> KYSKRIAWMKTTICDSLQLKDMIVEESFQYEKNKNLLEQFLSGEGLNKIFAYYQVQEQAQNDDIKDTGAQDPVLFFTTGDLEKIQDKAVWFLRITNPADDKKKASQQDGNDNDIIFGEITPNTVPMLNALMESVYSRQIDHIITEKIQFWGVAEEEQVLEFQQHSNKFSSEVREAINLMSPGTEHFKLDYEAISGLSESEKMQHYEMKFNEWINLISSQLNDDSEVRKDEKDAGPATELIYWRSRMQKITNWSEQLKSKDFQIVKASLQRHKNHDNQRPRGDESLSKLMMEYNRLDLLLTDKLNEAKDNVKYLTTLEKFIEPLYNGTPQQIIDTLPALMNAIKMIHTIARFYNTTDKMTGLFIKITNQMIKNCKDRILNKKDNGDNPSLYKMIWEQDPAELIEVLGSCIKLYCEYKKCYNDTKEKVADMPKGKTFDFSDAQIFGKFDTFVRRLQKLIEIFSNIQQFNALAKHNLEGMDVLTNKFKKIIDDFKKKGHNLLDTANNKFDRDWVEFNVEISHLDGELQNFIDNNFNRFRNIEYSLKLLHKFQSTIKRDSLKHNLTSRYNAILHNYATELDTIQRVFQDQKSNPPLVRNMPPEAGKIIWARHLFQKITGPINIFPENVINSTEIRRYYGSYNTLGKQLTIYEMWFYQDWVNKIEQSKAALQATLIVRHDENKKLYVNFDLEIMQLIREAKCLDRQGIEIPESARIILLQEDKFKTYYNELLYALKEYERINSKIKPICKNLLLPHIEDLDLKLRPGMVTLTWTSMNIESYLYYVHQGLKKLEQLIINVNDIIENRIENNLKTVSKVVLVHLPQDTKPLSLDSFVQLQEEYINSKTDFLTSKNVEVERAVDDLLQTIMLYPLDPHVDPVLPEETKRIKRYYFWYFYQALLNSTQNSLNAMKYRVCGKKIPGANTLQNLKPFFQVEVQLNGDKVTLNPSLQEIQKSINRAATAVLRCSKHLYNWDQQNKDSTDKATFYDMIACDKEIVKVILLLTGSIQGTKNKVNEFLSGFTKFEWLCKESIQESIKKFSKNGPTLQNYEDQLKKFSQIEEEIEKIVPTYKIGAMELMTHNICTSLSTWAKEWKLQYSQDLHKRARQLLDSLTEQTKMLSTKLSKPVKDIDSLGYVMETLEQIRKEQAEIDMKFNPVQEMYSLLDNYLPGGITDKDEMDARSLLRRNWDILIQQAEIKGKEYQHKQAIYLKELKQSIKDFTNQVSIFRRDYEKNGPMVEGISPAEAMERLRRFEDEYDVKYQMYKINARGENLFGLQNQKYPELEKTDAEIKNLNKLYNLYDSVIKNIQQFKEKSWQDVSKDDLAKMEEDAGKYGEQCSRLPKDLKEWQAYRDLKNYIDSLREQLPLIISLKKPSIMPRHWEKIKEITNTKLNYENPDQFYIEEIMGAKLLDFREDIEDITESADKQLKIRTGLDEINLYWNDMQFQFGIWGKRDVPCMLNGLIVGTILERLEEDQLQLSTFNSQRHVTPFKAEVENLIRTFSDVNDTLDMWVKVQKLWTSLEPVFTGGDIARQMPLQAKQFQGIDKNWMKIMEKAVETKKVIPCCQNDMLKDFLPDLNRKLEDCQKMLEAYLEGKRKKFPRFYFVSNPTLLKILSQGSEPTSIQEDFEKLFDAITKVTFESAKDKKNPALKQITQIQQVIGRNEENISLTGYYVKCEGNIEDWLKKLEQNMQQTLKDIASAAAQQVFQVGLKEFVSSQASQIALLGLQILWTSKVNEGLERLSRNERNAMDIKRNEIKEHMNILSSMCLEDLNGAVERTKVETLVTIQVHQKDISMDLKCKDVNDFEWQKQTRIAWKTDIDECIISITDWDSPYSYEFLGAKERLCITPLTDRCYITLAQAMSMYYGGAPAGPAGTGKTETVKDLGRTLGVFVVVTNCSDQHRYRDMAKIFKGLVQSGLWGCFDEFNRIDLEVLSVVAMQVESITTARKQHMKKFMFPEEEIEIELIPTVSYFITMNPGYAGRQELPENLKVLFRGVSMMVPDREIIIKVKLASVGYLQIDLLAKKFNVLYRLCEEQLSKQRHYDFGLRNILSVLRTAGNTKRQEIKSDEEMLLMRSLRDMNLSKLVADDIPLFNGLLADIFPKLKEVPKKLYPDVEKKIPEEINAESYLINTPSFQLKIIQLYETCLVRHGFMLVGPTGSGKSTIMKILTEVLTKLGSPHKIVIMNPKAITAEQMYGVKSEISDDWIPGVFSTIWAKSNNRALKHTTWITCDGPVDAIWIENLNTVLDDNKILTLANGERIAMTENCKVVFEVENLNNASPATVSRCGQVYVSPTDLGYEAVIEGWIRNRKASGRAEESDKLGNILRKYLINMRFIELQSKECKEPMMDTSPVISVINILNLLTGCLQYFVQTQRTLSEQEYEKFIVYSMAWAIGGIYEAQDRVRFHELLLAKNAPIPQKGKENETVFDYYVSQDYLDWKICSPEEWVPPQSLQFSQLLLPTLDSFRAEMLLNFILTQPKSHTCSNSALLIGGSGTAKTSSVLLYCNKFDPQKMLFKRTNFSSATSPFMFQSTIEAECDFKVGKEFAPPGNKMMTIFIDDMSMPFVNKWGDQITLELVRQLIETGGFYMLDKTQRGNQRKMKNLQYIGAMNHPGGGRNDIPNRLKRQFFIFNMILPLSIEGIYGPIIKHMFKQKYFSDSTYKVIESLTSATIALWNKVKSTMLPTPAKFHYVFNMRELSRIFKGILTCKKDTINDAPKSMKIKPELFLVGLWRHEAERVLADKLVNNKDKDTVMGYIQEVSLESFSQIENEILEKYSSEKTFLFCDFLRPDVINEDGIIEEEAPKIYEAIDSLTELRKRCNFLLSFYNDRNPSKKMPLVLFDDALKHLLRISRIIRQPRSSGLLVGVGGSGKQSLTRLAGFIGKNLIQQIIVTKTYSDKDLKEDIKKGFDDAGHLGKQVTFLMTDSEVKKEEFLEYINMVLSTGEIPNLLAKDEREVWLGDISQAYCKEKNLGNIDPPQSELWTYFVDRVRDNFHIMLCFSPVGQKFRERARKFPALFNECTIDWFLPWPEEALVSVAETFIKNFDKLDTKEETKQELMKHMGNVHLMVNEICDEYYQKMRRQVYVTPKSFLSYLNSYKTLYIEKYDELDQQEESFKIGLNKIQEATITINQMEISLKEEEIQLNEATEKTNQLLANLDKESKKANQKGEEVAATNKQCEIQAEQISKEKEEAERELEAALPALRRAQEAVDSIESKDIVELKANKKPLDIIKYIMNAVLVFFKARLIPIQIEERVFNKKEGKAVLFLKESYDESGIQTLGDMNFMKKLKEFEKDSINEETIELLEPYLNQSEDWFNDTFATKASKAAAGILKWAFAIYEYHQKSKIVKPKRIQVAIAEGRQAIALKELEKAREDLAQIQAYIKNLKDVYTKQMEEKNELEMKAAKTKKKINTARTLITSLSGEKDRWGKGAQDISDQKRKLVGNVSLSTAFISYCGPFNAEYRNKLAQQRFVVDMKKRGVPVTPGLELTSFLIDDATIGEWNLQGLPKDDLSIQNGIMVTNSARYPLFIDPQGQGQNWIRNKLSASIIPERCITTLSHPKFKDMFLKYCMESGLTLIVENIENEVDPMMDPVLERQIIVKGKTQFVNVAGTEMELSKEFKLFMTCRLANPSFSPELSAKTTIIDFTVTQSGLEQQLLGKVISKEQKALEDSLNQLLADVNQNQKDLQRLDKNLLERLINSQGNLLDDTELMDVLNNTKTQAKEVAAKLIDAEIKTKEINEKREQYRPVAIRGSAIYFTMIEVSLVNWMYNSSLEQFLKLFIESIDLSEKAQLPSNRVKNIISFLTFHVYRYVNRGLFEKDKITFILMMAFKILTTAGTISSGDVSLFLKSGDALDIKSERQKQISYLEDNQWLNILALSKHTFSGQTLPFFKELPDLISRSENQWRNWIDKNDPENFPIPDFAESINQEKEIGSFISLCLVRSLRNDRTLIATQNFISNVLGKEFTDPISYPIEGIWQESSNMDPVLFLLSAGADPTSSIDELAKKKKKFPCEKVSMGEGQERVARQVIMKGFVEGGWVILQNCHLGLKFMEEIETLVSPINQIHEDFRLWITCEQHPKFPLGLLQKTLKVTNEPPKGLKAGLYKTFTTIITQEFIDKVDHSNWRSLIFTICFLHSIVIERKKFGPLGWCVPYEYNYSDLEASLLYIEKYLTNLMSTPQPNSHNLPISMNVVRYMICEVQYGGRITDDLDRELFITYGETYLKDGIFGNDYFFYDIMVDGSGQKFKYRIPQNPSAELIKYQEYIAKVPTVDNPEVFGLHSNADLTFRLKESKEMINTVMETRPKDSSVGGGKTREEIVQDKAKDMLKNLPPDYNDVEVRELVSKLGGPNPKTSTERGMTVPLNIFLYQEVTRMQRVIGLVRKTLQDTILAIDGQIIMTPEILEAINAIYDAKVPNSWLYDPSGAEISWLLPNLGSWSTSLSDRNKQLNDWLRSGQRPILFWLTGFFNPQGFLTGMKQEVTRNHKKGDGKGGEAWSLDDVVYSTTVKEREKEKDIEQPPAEGVYIKGLYLEGCKWSKNGLDDSDPKKIFADLPILHVSAINKKKTNEQDRMSNTYLCPVYKYPKRTDKYLIFRVGLPCEGSNNPSHWKLRGVALLCST;> MGDHSQKDSPEDFIINRLSQALGIQKEKIKKSLETAQDDKGEVTNKDEFQGFIQQDNSTNILWVSGQSEKCTFYYGQLPPIDKFKKKGIAVIKLGLHKLTNENVAKDVVVVEITNNLLEHLNSVFNEIMSPVMQNPLNQQGWTDLVAKDLMEKFNNYVAQVYVLLGQIKGKTMLPLPSHKLTSSDTTPDKDKAHVFEGSIITWTKQIKNVLKLEPEQLLKYGNDPGPLAEIEFWQNKRDNLNLIDSQLKSVEVQNILHFLDNNKSTYTTPFTKLQAEVKKARLEANENYRYLFTLKDLFSKLQESQPSDFPTLYELFIPIMHTILLIYNKSKTYNQPPRLVVLIREICNAIISNAQAFVDKDTIFSLIDSKETTEACDKLQVTLDVCSKFKDAYFEYKAKAGGNWKLTSNALFVRLDSFLERCQDILHLTNTIVQFNKLEKIELGGTKGKTLTESIAQIFKEFEEAVQAFTSVSYDIMNIAEKKFDDDFYEFRSKIKELERRLASVITQGFDDYDTIYGRFKLLDNFEGLLTRPIIADELEKKHIVLLEMYKQDLKQVQSIFLEGKQFVDSMHENAPLFLNMPPIAGALTWCKSLRDRIQEPIEKLAQLGQGITEREEYKDVQKLYTSITKSIKDYEDQKILSWEKEVEDSSQDKLKQTLLCKDENDLIKVNFDPSLVRLLKEVKYFLLLRLEVPTTAKDIYTKAETYRTQIVALDMIVDNYNHIKTCLLPVEEPLVKKKIQDMEEEVKPGIEEIRWKSTNIDQFISKSKSIVDQLFETVNKMKDSLQKIHKSLANFNVKIIERKNRPMSPDDYDQFLKAIFSNKLTIVKDNGNQIQKLVKEVLDAVKADKKQNSWKNYNDYVNVIVIEGISTAIQTALLHLNEQINPVFIKRNDISPLFDIRLELGQSGIQFDPEIGESSNQLTVRNTIRNWINDFFNIAGTIQRLDTTMPGDFLQEIRSFFEIKQCLAMITQNLEWIENECNQFRARFDTYSYLWTEDEQISFNRFLDENEPKDEDGKGGDDDEGENTEKQNPLLKGCRAKIPNLDLFDEKITHLKAIQQEISRIKTPEDISWLRINLQPMKTALDARVTRWIRVYTDFLVNQFRTTQKNLLDFIEKTKDGIKKNPADHENLHDKKLLMSVMKVISDVKDVEPRREGIITRMKEMVTKLKKHNVPITEKGTDDPLQQIDNANSNFIEIYGRVFKVKADIIPLQAEETQNIKRDLDIFMKEVESFRKEFMQKLPFDYTESMGYENINNAYDTIMVYYHKLTAIEGRALEYNNLEKAFELQKSNYKQLKDCMNDLKNLKTMWDAIALIHFQYNDWKTKPWRQIKADILLDTNKTLGTQIKNLPKEIRNFKGYNVIVEKVKNMGTVLPLVSALHSEFMEDRHWSQLKQITGTVFDHNSLSFYFEDILALNLYKYENTVNEIVDVAQKEAKIEKKLKNIEQWWSKQVFEFTEYKETKTFASLDNMMEVLDQHSLDLMGMKSQGKYVEFFYDRVEDWREKLGRVDVVVNEWLKVQKNWKILYNIFLLSEDIRMQLPEDTKVFEGVDKEFKDMMSEVSANPSVVEACTIERRDVLVGWSQAIKKCEKALNDYLEQKKKSFPRFYFLSNQSLLTILSNGQNAPKVCEYLGDCFDGLKTLTFEPPANPAETSKVGIGMISKDDEKVPFSSKFICEGAVEHWLLNLEFRMRETLQEILEGAKNTADLWDSGDKPREEWVEGYNAQIALLTTTIVWTEDVGRAFEDLAGGSETAMKECQKLIEVRLENLIKKVRGDLHILERWKIINIITIDVHSRDVVEKFVIQKVSEAESFAWLSQLKFYWENKPDSDMHLRQTLRFPWEKDKNKNKCIIRIVDWFRFYSYEYIGNAIRLVITPLTDRCYITLTQALNLTMGGAPAGPAGTGKTETTKDLGRAIGIPVMVFNCSDQMNKDSMAQIFMGLSQSGAWGCFDEFNRISIEVLSVVSTQVKCVLDALKEKKTKFSFVEEGEIQLQDTVGFFITMNPGYAGRTELPENLKALFRSCAMVVPDLALICENMLMSEGFTMARVLSRKFVSLYMLSRELLSKQKHYDWGLRAVKSVLRQAGKLKRGDPDMPEDPLLMRALRDFNMPKIVTDDKVIFRRLIGDLFPKLDPPTKQNPELKKIVQDTTKKDMGLVAEELFVTKVVQLAEILEVRHCCFVIGPPGSGKTCVWKTLIKSYINSGEDAEYDTLNPKAVTSDELFGAYTKTKEWKNGVIAVIMKNQVKNEEKYKATHMHKWSVLDGDIDPEWIESLNTVMDDNKVLTLVSNDRIFLTPQMRLIFEISNLRNATPATVSRAGVLFINETDIGWMPYMNSWLERSQINILKQQKEMANMPEYPVIDDVAKSVFYRCFQSYFEQNIDVHDKNRVRHICPMVDIAMIQTICTILDALLIQHLPKLKQMKEEDEKQALEAFFIFAGLWAIGGPVGGGQDDSKDMKEFNTVWKGAAKVKFPEQGLCYDYYYDINENKWNTWKVEDYLPNDQPLFSKIYVATIHTTRLRYMIDIHLQRRKPILFIGSAGTGKTAVVRDYLNSTRPEQVSHKTINFSSFTDSLALQKNIESMVEKKNGRNYGSATNKVLICFIDDFNMPYVDKYGTQSPIQLLRLILDYGSIFNREQLEERKFLQDLLFFGCLNQKSGSFTVDLRLQRNFSVFSMYTPSSDVIKTIFGSILNAHLSTIDDKAQKMAFKLVEATYFTFDKILKNTTAFAPSAKRFHYQFNFRELARVCEGICRTTPGQYSGGDQGKLVRLWAHEMKRTFEDRFIANEHVEFFRRYLTEAISKCIGEFPETENPIAEPLIFTGFVAAHQGLDQQYTQCTIPVLKRVLDDKLEEYNEVKAQMNLVLFQQAMEHVSRICRILDMPGNNALLVGVGGSGKQSLCRLSTFINGFEIDQLVVTASFTINDLRNNLQEIYKKIAKPNSIARVFMITDSQIKEEQFLIPINDMLNSGWIFDLFPKEDMDSLVSGVRNEAKGEGVDVNNLTALTSYFLDKIRKNLKVVLCFSPVGDTMRIRSRKFPGIINNTSIDWFHPWPHEALIDVAFRFLEEIEFPTEEIRQSISLNMAKVHSSIDTANEKFLKLERRYNYTTPKSFLELIDFYKKLLTEKRETIQRQIQRYEMGLNILAETQNKVQGLQEELKVKMVEVNKQREETDILIEKVGKESALAEEEQTIANAEEEKTNVAAAEAEKISKEATEALAEALPALRSAEAAVDCLKKPHVTEMKNLGSPPAGVIVTARVVLILFNQGITLNDPDEKVWKKAVTFMNNPQAFIDKVKSFDGENIEPNIIEQSNKIIQDPSKKFNEKDMAGQSYAASKLCAWAVNIVTFNKIFKQVKPLQDAQKQANEILEEKKKELAIVKQRVAELNARVNSLKRQLEEAEARKMIVEQDAARCQSRLSAAENLVNGLAGENKRWTQNVKFLKENIKSMIGDSLLASAFVSYIGAFSAKLRLELWKNTWLPDIIEKGIPITEGIEPLKILTTEAIKSKWKNEGLPADPMSLENAAIITACARWPLIIDPQLQGSTWIRGKQGENLTTISLSQPKWLGALTSSISSGRAVLIEGIQQEIDATLDPLLQRAVKKNGNQLQLEIGGDPIDYDPNFKLFLMTKLINPHFRPEIAAQCTIINFIVTESGLEEQFIAMVVNIEKNELEMAKQDLVKKQNEYAVTLDKLESDLLQSLSEADPATILDNTELIQNLDKTKKTTIEITEQQQKAKVTEAEINIQREHYRVVAAEGSMLYFLVISLSVMDHMYQYSLESFITFFFKAINRTTVRDENRIPTLILNIRQTIYQWISRGLFEKHKLIFLTLIVFRLMQKKIIDVAYEVAEMDFLIKCPARPGVENTLDWLPNISWDQIQGLINLEEFRNFAHQLEKEAPNRFKDWYNELQPEDQKLPLDWKRLDSMPFKKLLVLRCLRPDRMTISLNNFIRAVLPQGDAFVEMDQKLAFSEILESVINEDAESTIPIFFILSPGSDPVKEVEKIAKKKRIEPGKNFFNIALGQGQDEIARRRIEEGNKEGHWVMLQNIHLMPTWLIELEKILDSYSGEAGGGNSEFRLFLSAEPSTGIPIGILDRSIKLTNEPPAGLKANMKRAWTYFSKEEIEDKDPKIKSILFALCFFHSTLIERRRFGPKGWNMSYPFNMGDLRDSYLVMNRYMEQNQGGKVPFNDLIYIFGEIMYGGHIVDDWDRRLCNSYLFNTMHEQLFDELELFPYIEGKGLSFKVPGQNPYEKYIEHIETSLKQETPLAYGLHPNAEIGFRTDQCKTLFNTLLELMPKEQSRDEKSSDIKSSNEMASDLIKQLLEDSELKNKIFNMEEIKNKIDAENKGPYQNVFLQEIEYMNALLSEIVKDLEEIGQGLSGLLTVSENMEMIIESIALSRVPASWQKLAYPSKRGLQSWLANLFQRIEQLNIFRDDPYSIPRVVMISRFFNPQSFLTAIMQVISRAKAYELNKLYIQTEITKRSIEEIEGAAKEGAYVYGFILEGARWDYQLGQLEESKPKEMFSVLPVTYCKAIPLPPEGKEDKSLYQCPVYKTEDRGNTYVFTAQLKTRFPPRKWILAGVAIIMDVEGVSD;> PLVWTQLKQTGTTQPTARSGHTIITVGKTHIMFGGLDNDKNNYKDGKIAPNNQVFTLKLTQNNCEWRQIACQGDVPLPRCYHASCAISADKMLVFGGSYTSNLRFNDTYILKTTSYQWSKPANQISGGEPKNAESKIGAPQPRYGHSATFFEGKVYIFGGHGGINYQRLAFNDLYVLETENFEWTRLEPKGNPPDPRGGHSAAMMANKPQLMIFGGWSFTSQYSNIMIYDIEKDEWVDPEIAHEIPKWNLSGIMAPSIPSWKYFIFGGSVGSFEEGGNRTNSRFVDDSFVLDIDTLSWSSINLEADETSKAVCKPRPRESASIFYDSGESRAIVFGGWANNWLNDLWALNVSTITGPPIFSIKPALGPLTGKTKVLIEGDGFKDTQNISVKFSGGKLEKEVNGTFVNEKEISCETPTFDYPRSVEVTVCMNKGDYTITKSAFTYNTKADKTIAYGPGLLTENLIGVQTTIVIQARNGSDEFVVTIRNPAKIKKEEEVKEGDKANTKNTIKEDEEEEGEDEEENKKKKEAEKNDLTGSAVMNYISKQLKDIQEFIENTKENIEIRNKNISELINVMINLEKVRVKNDDDVLTLDTVEEMLNFLKKKKDSDIKKCKKLQEEWKNLAKMAQAVKKDIQNPVKTESDKTKENIKKFEEITLKEYANSLKKESFFIYKTGVSESFKRIGEVKQKVDEFEVQLNQYEDFARIGSKKLMEQIRTDVSSVEKLWVRIEISEKTMDEYKKMKWGSINSMDMEDEIKKLRKALTDLRGIDKRSNAFIGITEELKKWATFLPLLGELKDPSMNSEDGRHWKKLKDLVKKEFDVSQELMLEIIWDLKLFDYKDGIEEITDQAKQELKMEKALKKIIDFWRDIEFELVQHKNTDIHTLKMSEENFETLEDHQLQINNMLLSKYVAYFEKEVEKWKYDLGSVYDVVQLLLEVQKTWSFLENLFEVKRELPNESAQFVGIDKDMKEIMQKGCDIKNCLKFCTIEGMLKRLENIQAQLKVCEKALNEFLDSKRRAFPRFYFVSVNDLLDILSNGNSPAKINRHMSKIFQAIDNLQLKEDSSGGRPTLKMISCVGTEEVDFSSPRLLQGKVESYLKDVIDTMIGTLKSVANSSFKNFQSMTRKEWLKSDPSQITLLVNNIIWSKAVEDCFLKLQSGDINAMKLFLDESIKQLTELIGMVQGDLSKPLRQKIMCLITIDTHSRDVVHRLINEHVRKAEEFQWQSQLKFYWVDNDAKIKIADARFVYNYEYLGNGPRLVITPLTDRIYVTATQALHLKMGCAPAGPAGTGKTETTKDLANALAKACYVFNCSSEMNYESMGNIYKGLASSGCWGCFDEFNRLLPEVLSVCSVQFKAVTDAIKQNVERFIIEGDEISLDPTCGVFITMNPGYLGRAELPEGLKALFRPITVVVPDLELICENMLMAEGFIEAKILAKKFVTLYMLCRDLLSKQLHYDWGLRAIKSVLVVAGGFKRSEPEIAEQALLMRALRDFNIPKIAFQDLYVFHGLLGDLFPGINIKPKKDLDFEKIITDVCIENKLDPDPEFVLKVVQLSELLAIRHCVFVMGPPGAGKSTTWKILAKAQDKTNKKTTLIDIDPKVVSTKDFYGYNLPSKEWKDGLFSKMLRSLAEQPDTNPKWICLDGDLDANWIESMNSVMDDNKILTLANNERIPLKPHMRALFEIRDLRFATPATVSRAGILYISDEVGYQWRSYVKSWIKQEFSQDQEMSKNLDTLFGKYVPDTLDHIKKHCRFLVPVSPISQVISICKSLQTLLKGDVKNLEYLFVYALIWAIGGALAEKDSIDYRKDFSTWWKGAWKTAVKFPSKGTIFDYYVDQSGDSSKFVEWSKRLENKEFDPQVETMGNITVNTIETLATTEFIKSYLMVKHPSLLIGNSGCGKTQLAKGILKEIVQAKPENYAYQLINFNYYTDSTYLQGQIEQTLEKKAGRQYGPPGKVQLIYFIDDLNMPQLDAYDTQTAIALLRQLADYGHFYDVSKLALKDIINTQVLAAMNPSAGSFFVNPRYQRHFWTISIPFPDNESLSLIYITFLNGHLKRFKSTIQEYSNIIVRASLMLHQAVTQNFRKTAINFHYEFNLRHMSNVFQGLLLSDPNKFTEPDKLIKLWIHECERTYGDRLVSTDNLKTYKENIFDIVKKSFSKFNFSRYFGNNPENLIYCNFIAGINSDRFYDQMPNNEMEKHISEALKEYNDNNAFMGLVLFEDAMKHVCRICRIVLPSSGHALLVGVGGSGKQSLSKLASFIMGYTTFSITISATYSMVDLRNDLQQLYFKCGPKEEGILFLFTEGQITNERFLVYINDLLSSGEIAELYTLDEKEAMINQVRAKVKGEGKPDTRENCWNWFIDQVKKNLHMAICFSPVGDMRRRARQFPALVNCTVIDWFQPWPYEALFNVAKSFLEPVDLGDDKVREAVVKFMPFSFTLVNDLGLKLLEQERRYAYTTPKSFLELISLFTNMLAQKRESLERNKERYETGLVKLKETAEQVAIIEVEVKEKQVEAEAKKKEADAFAEVVGREKDKVEKENSKATIEADKCGLIKQNVEAQKSSTQQDLDAAQPLVEQAKSALNSISKKDFQQAKSFASPPAGVPEVFAATIYLLAGYFNEAIEIDKNKKPKDVSWKSSLKLMKSPEEFMEKLLNFKDVVDANQVANVNIVKNQYLNMPSFTPEQMASKSAAAKGICSWVVNIVKYYDVIQDVEPKRKALKEATEQLEEATVKLNEVEEVVRKLNEELNKLKAENDKAIAERNAAISEAERCARRLNLAQRLVTALSSENERWGKSIIQLEDQLKLMVGDVLVASSFVSYSGPFNKKFRNIMINQNFMKFMKEHTIPMSPDPNPIKILTDESTIALWNKQKLPSDSVSIENGTILTNSARYPLMIDPQLQGITWIREKEKANNLKILRLGSKNINRDLELSIENGYSAIIENMNERIDAILMPIIARSFIKRGKNKIIKFAGKDLILHPNFKLFLHTKLSNPHYPPEIQAEAALINFTVTEAGLGDQLLSLVVARERPDLAKMKIELITQQNDFKIKLKDLEDELLYKLANAKGDILDDIELIENLEYSKKLSVEIAEKVAAAKITEAKINETSENYRPAASRGALFYFLLSDLSKVHSFYKYSLESFIVVINRAIDAISENKIYGKTTMMSPRSLKKRVDELIESLTYTAYQTTRRGLFESHKLIVAAMLCLRVLLRSEELNSDEVDHLIIGKVDVNPTPMPDALKSFLNDNIWAACKALETIHQFQGFCQSLETDVLQWKKWYSEEKAETADLPKAFKELSKFHRLLLLRALRPDRLPSALSQFVHDKMGERYIEQPPFNIFETFQETSKTVPIFFVLFPGVDPTPDVERVAATFDVSANNGRFINISMGQGQEDRAKKALFDCAQKGHWIMLQNVHLMQSWLYGLNGLEGFLESVFASPKTHPNFRVFISSEPPNVLLPLMQIIPESILQGSLKIANEAPQYLKANLRRAYNKFDQEFLDKCDKKPTEFKSCLFALCFFHSLMLGRKKFGTQGWSRVYNFNDGDLTICADVLYNYLSKYDQVPWDDLRYIFGEIMYGGHITDDWDRRTNRTYLKVLIRSELLQQNFNLAPQFKSPDPSKFDYEAYRKYIEEKLPIESPQMFGMHPNAEIGYLTQTCDQVFNTILEVQGGSSGGGASKKDDGVMVTLTDFKTRCPHDFNMLLIEEKVKEKTPYIVVCLQECERMNGLLKEIKTSLEDLRLGLTGALNMTDAMESLQQSLSFNKVPDTWEKKAYFSKKPLSSWFADLIERNIQLQEWCKELVTPTSLCISYLFNPMSYLTAIMQFTARAQGLPLDGITIQTNVTAMKGPEDVVNPAENGAYIHGLFLEGAAWEIGGQGQDGYLIEQKPKELHPKMPVINAVAVPLDKKKKNGQYDCPTYVTSARGQTFVFTANLNMESDDSDPNKWILSGTCMLMSDD;> LTAQELNEDMPSKMLEPKNPQAPKNITVYDYYTRKFKTDELVDQMIVHFSMDGDYIWKESNEYKTQEEIRDTKKALIKEAMRKQESEEPGANHDEEAIKQTLRNKFNYNTRECQTINPSIRERGVSTEPPPSDTICGNITQWEIFDAYYAEIMKDHQIENKKKKEVDQDKKQDQSMYSTSFKRCCKIMERMVVQNDQEDKYHDYRYYWSQGDNLEAGKNEGHLLPIWRFSNEKQRKKNVTSICWNPLYPDLFAVSLGSYDFTKQRMGLICLYSLKNTTHPEYAFNCEAGVMCLDFHPKSAALLAVGLYDGTVLVYDIRNKHKKPIYQSTVRNQKHTDPVWQVKWNPDTSKNYNFYSISSDGRVMNWILMKNKLEPEEVILLRLVGKNEEESTLIGLACGLCFDFNKFEPHIFLVGTEEGKIHKCSRAYSGQYQETYNGHLLAVYKVKWNNFHPRTFISASADWTVRIWDSKYTSQIICFDLSMMVVDAVWAPYSSTVFACATMDKVQVYDLNVDKLNKLAEQKIVKQPKLTNLSFNYKDPILLVGDSHGGVTLVKLSPNLCKSGPEIKQTEDKKAMEEFKNVKIEDYEREKMENL;> KEFNNPINFQDTETRYGGIQNQVVNINQYVQRNPNFIDLDNIAELSEHSVNTERVKTGDRGMSHKEGGWPGNVDPNEAQETGRFKKRIEKDTSFPQAVKDLKEGVEKCIYQNNQIDLLEEYFEGETSEHVVENLSSKTLMLFKDEKEICKRSVSEISWHPEGPTKVAVSYAIMRFQQMPEKMPTQAYVWDLLNPNSPEIKLMSPSAVTNISYNQKIPDQIGGGCYNGLLAVWDGRKGENPIMISPVENSHYEPVTHFHWLMSKTGSECVTTSTDGKVMWWDTRKFEAGPVEKLNIIEGLGENEEIIGGTALEYNVEAGPSKFLIGTESGSILTANKKLKKPVEITTRYGLDQGRHLGPVYSINRSNQNPKYFLSVGDWSCKIWVEDLKTPIIRTKYHGSYLSDGCWSPTRSGAFFLVRRDGWMDVWDYYYRQNEIAFSHKVSDSPLTCIKINQTGGAYHNSGKLCAIGDQDGTVTILELCDSLYTMQPKEKDIINEMFEREYRKEKNLETIKKQQELAKRQVQKDMGSQKEKWEKKKLEMIETAEASFHENLAKNPV;> NADDQLKQLSALEGANGYVIFNESGIPLKRHEKSISHEKAVHIAALVSDLWNVSKKVIQRDLKTPENDIEVIRLRTKHSYEYIITQSGDFTMLAIQLCGKAIEEAKKAAAAAAAAAVVQEENKEKEKK;> IYKTSKEIQKSDQRIIQQRVENSIINNQIYQKSLKRKTSKRKVRHQANKKNFQKEMSEVEDTLNRIKTHKTVLGYLIVNSEGGVVRGAFKDEEESKNIANSIPLLTKKARSVVRDLDPTNDLVFLRIQTKLNEIMVAPDDEFSLIVIQTKG;> SHLDKVQPVIKNSDMSVEMQKEVEEVAKKAIDYCNTDKEIATFIKDDFRSRYHGTWHCIVGRNFGSFVTFERSYYIYLYVGQLAILLFKTG;> KAVTDMDINELRKLMIGKAIINSSDMQGDLLQEAQDVIQSGIENNSAPVLNIEAACKYIKENLDKKFGPTWQCIIGEGYAYDVTVQNNTLLFMFYNGNLAVLIFKS;> QQYKTFMGARVLWPPECADDILEGAIRETQDALKKFEIAREGQKIAEHLKKYMDDHFDPYWHVFFGKNFGCQAVHNKNRFIYFYIEKTAFLMYQT;> HANEQIIDMPENSEMKSMKNDAFSQAKFAVENYKFENKISSHIKKFFDEKYGPNWHCVVGKHFNAYVSYDSKNFIFFYEGQLAILLYRKG;> MSDSDSDEGRVVEEPLPPHIIRFNDMAQHLLKKVIRQADVLIKENPQGLEKDIALNLVKFVKSQPEFKIGDGEWQCIIGKNFGCSLTFDANVLAFFDLLPSRKSILLFKSG;> MNHEPEVKATDMEEDMIKRVKEIAINAVKEYKQEKQIAHYIKYEFDKIDGYGWNCIVGRNFGSHIIHQTKKYIFFKINELCLLLWKA;> TDKEYISEEVQKAIDDSVKQVFGIKDDSSQVTITYNKDKVNLWTQQIIDYTIRGLNKLGKHFKYCVTAILQQTNHAGISVQITAYQDTATDGSLIQCYEINDIYAIVSVFAMAV;> RKREASLITLNYIKNRFYPSKIQKIIKELFEDRLKGVEYDPNNANQLSERLVLELREKIKRGKVPRYKIGVQVVFGEIKGQGLRIASKCLWDVQNDNYASYTYTSEKVYCTGIVFGCYFE;> TTTVTSEDHFMTFYNENNKKLIVVDVYPGWSGPCTAMYPTYNQLMISIDDFEKRIDILLLDQDKLVTYKNDKFHATCQPKFLFISEGKIIDEVLGTNIPVFIEKVNKYIPLS;> AKGTTCQKAIVNWEAANPGKNPSEAEEIKLIFQIPPIEKMDGPVLNTLTKCKKLSLSSNSIDKMISLNMLRNLEILSLSRNVIKKISGLEDIGGTLRQLWLSYNFIEKLDGLNNCSVLQTLYIGNNRIKNWEELDKLKDLPELENVLFYGNPIYEQVKEDPKLIVLKKLPTLKNVDGMIIDDSVLEKVKQIA;> MASEVMNLSEEDIQFCQKAFSDYDEDGLGAIKVSDLKLALENIGCSLSENDLFKMISEVDEKNTGLIKFSDFLNIYYKQKYANLGDDDQDLVDAFVAMGGNADTTGSVDANRLIQIVKEEFEMTIDIVGLIREIDKDGSGEIEYEEFKLL

Thousands of outer-arm dyneins (OADs) are arrayed in the axoneme to drive a rhythmic ciliary beat. Each OAD is divided into two regions, a head that contains AAA+ rings (rings) for ATP hydrolysis and a tail that holds together the whole complex. The tail is permanently attached to the MTD A-tubule, while the head region of each HC contains a microtubule-binding domain (MTBD), which binds and releases the MTD B-tubule depending on the nucleotide states. We reconstituted the purified OADs onto MTDs to mimic native arrays and determined the structures, by cryo-EM, of free OAD and OAD arrays bound to MTDs (OAD-MTD) in two different microtubule-binding states.

Cryo-EM classification reveals that the OAD arrays adopt two distinct microtubule-binding states, MTBS-1 and MTBS-2. In both states, the relative axial positions for α- and γ-MTBD are fixed on MTD (γ-MTBD is always 8 nm ahead), while the β-MTBD position is equivalent to either α-MTBD in MTBS-1 or γ-MTBD in MTBS-2. The OAD array is dramatically remodeled when β-HC moves one step ahead from MTBS-1 to MTBS-2, coupled with five major structural changes throughout the entire OAD-MTD complex. First, an 18-degree rotation between the β-stalk and β-MTBD is required for microtubule-binding state alteration, whereas β-MTBD remains in the high microtubule-affinity state42. In MTBS-1, β-HC adopts a post-1 linker docking mode, which is precisely switched to post-2 along with β-MTBD stepping forward. From MTBS-1 to MTBS-2, the α-linker docking groove on β-ring is also switched from groove-1 to groove-2. From MTBS-1 to MTBS-2, LC3BL takes over γ-Ig-PT to contact β-AAA4L. Fourth, the tail of OAD is rotated downward with respect to the head from MTBS-1 to MTBS-2. Comparing with previously reported dynein structures reveals that the ADP-bound state43 has a similar linker docking mode to post-2 of β-HC. Therefore, the β-HC in post-2 probably mimics the state after one complete nucleotide cycle.methyl ({5-[4-(4-hydroxypiperidin-1-yl)-2-phenyl-1,3-thiazol-5-yl]-1H-pyrazol-3-yl}methyl)carbamate | C20 H23 N5 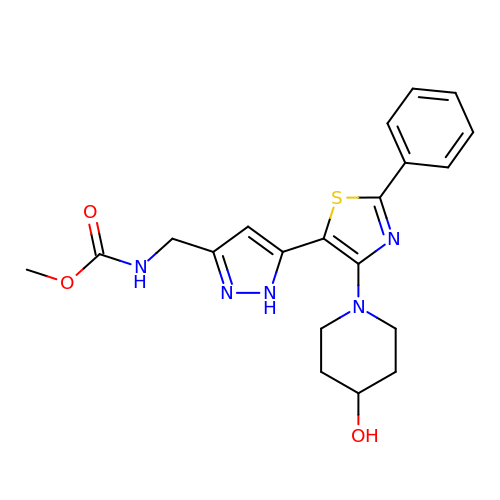O3 S | GFUMDRBVYNGSBP-UHFFFAOYSA-N> GSHMASMKKKGSVVIVGRINLSGDTAYAQQTRGEEGCQETSQTGRDKNQVEGEVQIVSTATQTFLATSINGVLWTVYHGAGTRTIASPKGPVTQMYTNVDKDLVGWQAPQGSRSLTPCTCGSSDLYLVTRHADVIPVRRRGDSRGSLLSPRPISYLKGSAGGPLLCPAGHAVGIFRTAVSTRGVAKAVDFIPVESLETTMRSP

The HCV NS3/4A protease – a chymotrypsin-like serine protease – is a prime therapeutic target that cleaves four known sites along the virally encoded polyprotein. The NS3/4A protease also hydrolyzes two human proteins, TRIF and MAVS, which are part of the innate immune system, thereby confounding the innate immune response to viral infection. In this study, we report that four chemically representative protease inhibitors – telaprevir, danoprevir, vaniprevir and MK-5172 – exhibit distinct susceptibilities to the protease variants R155K, A156T and D168A. To elucidate the underlying mechanism by which chemically diverse inhibitors bind to the wild-type protease and drug-resistant variants, crystal structures were determined for 16 inhibitor-protease complexes. These complexes include wild-type protease and resistant variants R155K, D168A and A156T each bound to telaprevir, danoprevir, vaniprevir and MK-5172, with resolutions ranging from 1.10–2.50 Å; S139A protease variants were used except for telaprevir, which requires covalent bond formation with the serine 139 for efficient binding.

Notably, MK-5172, though active against the other two variants, lost significant potency against A156T (A156T IC50 = 108 nM). A156T, the worst of the resistance mutations for MK-5172A, sterically clashed with the P2–P4 macrocycle and caused a large shift in the binding position away from the catalytic triad relative to its wild-type structure. This altered binding of MK-5172 resulted in fewer van der Waals contacts with D81 and R155, and is likely responsible for 1000-fold lower potency against the A156T variant. Overall, analysis of the four crystal structures explains MK-5172's significantly retained potency against R155K and D168A as well as its loss of potency against the A156T variant due to the rigidity of the macrocycle. Similarly, vaniprevir and MK-5172 exhibit significantly lower potency against the A156T variant due to direct steric clashes, while danoprevir partially accommodates this steric burden by repacking against the mutated surface. However, drugs such as vaniprevir and MK-5172 containing P2–P4 cyclization likely select for the A156T variant due to the rigidity of their P2 moieties.>MSKKKFVIVSILTILLVQAIYFVEKYHTSEDKSTSNTSSTPPQTTLSTTKVLKIRYPDDGEWPGAPIDKDGDGNPEFYIEINLWNILNATGFAEMTYNLTSGVLHYVQQLDNIVLRDRSNWVHGYPEIFYGNKPWNANYATDGPIPLPSKVSNLTDFYLTISYKLEPKNGLPINFAIESWLTREAWRTTGINSDEQEVMIWIYYDGLQPAGSKVKEIVVPIIVNGTPVNATFEVWKANIGWEYVAFRIKTPIKEGTVTIPYGAFISVAANISSLPNYTELYLEDVEIGTEFGTPSTTSAHLEWWITNITLTPLDRPLIS[2x]

The hyperthermophilic glycoside hydrolase family endocellulase 12 from the archaeon Pyrococcus furiosus (EGPf; Gene ID PF0854; EC 3.2.1.4) catalyzes the hydrolytic cleavage of the β-1,4-glucosidic linkage in β-glucan in lignocellulose biomass. The hyperthermophilic archaea Pyrococcus horikoshii and P. furiosus have glycoside hydrolase (GH) family 5 (EGPh) and family 12 endocellulases (EGPf), respectively. The optimal and denaturing temperatures of EGPh are 100 and 103°C, respectively, and those of EGPf are 100 and 112°C, respectively. EGPf appears to be a secretory enzyme because of its signal sequence at the N-terminus.

Here, we describe a new crystal form of EGPf prepared at pH 5.5 and compare it with the previously solved EGPf structure. Based on initial screening results, high-quality crystals of EGPfΔN30 were obtained using a reservoir solution consisting of 100 mM CHC (2:3:4 citric acid:HEPES:CHES) buffer pH 5.5, 200 mM lithium sulfate, 5%(v/v) ethanol at 22°C. The average size of each crystal was about 0.7 × 0.5 × 0.3 mm after one week. This was a new crystal form with symmetry consistent with space group C2 that diffracted to 1.68 Å resolution. The final model contains two monomer molecules with 270 amino-acid residues each. pH5.5, poor electron density was observed for the loop regions of B3–A5 (Gly131–Asp156), B5–B6 (Thr182–Asp194) and α-helix–B4 (Ser272–Glu283), but the regions were interpretable. Comparison of the structures at pH 5.5 and 9.0 showed that the structures of both main chains are the same. Comparison of the EGPf structures obtained at pH 9.0 and pH 5.5 reveals a significant conformational difference at the active centre and in the surface loops. Glu178 seems to play a role in controlling the optimum pH of the enzymatic activity. In conclusion, crystal packing is weaker and the quality of the EGPfΔN30 crystal at pH 5.5 is lower than at pH 9.0 because of the flexible interfaces 1′ and 4′.>[2x]MASMKVAVLPGDGIGPEVTEAALKVLRALDEAEGLGLAYEVFPFGGAAIDAFGEPFPEPTRKGVEEAEAVLLGSVGGPKWDGLPRKIRPETGLLSLRKSQDLFANLRPAKVFPGLERLSPLKEE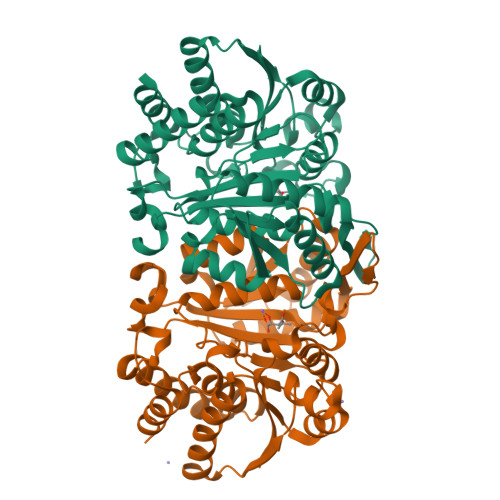IARGVDVLIVRELTGGIYFGEPRGMSEAEAWNTERYSKPEVERVARVAFEAARKRRKHVVSVDKANVLEVGEFWRKTVEEVGRGYPDVALEHQYVDAMAMHLVRSPARFDVVVTGNIFGDILSDLASVLPGSLGLLPSASLGRGTPVFEPVHGSAPDIAGKGIANPTAAILSAAMMLEHAFGLVELARKVEDAVAKALLETPPPDLGGSAGTEAFTATVLRHLAAAALEHHHHHH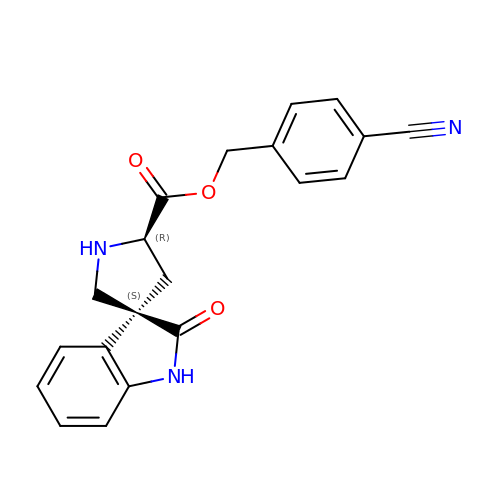4-cyanobenzyl (3S,5'R)-2-oxo-1,2-dihydrospiro[indole-3,3'-pyrrolidine]-5'-carboxylate | C20 H17 N3 O3 | QVGGPTMZUCXDDT-YLJYHZDGSA-N> MALLAEHLLKPLPADKQIETGPFLEAVSHLPPFFDCLGSPVFTPIKDVISGNITKIKAVYDTNPAKFRTLQNILEVEKEMYGAEWPKVGATLALMWLKRGLRFIQVFLQSICDGERDENHPNLIRVNATKAYEMALKKYHGWIVQKIFQAALY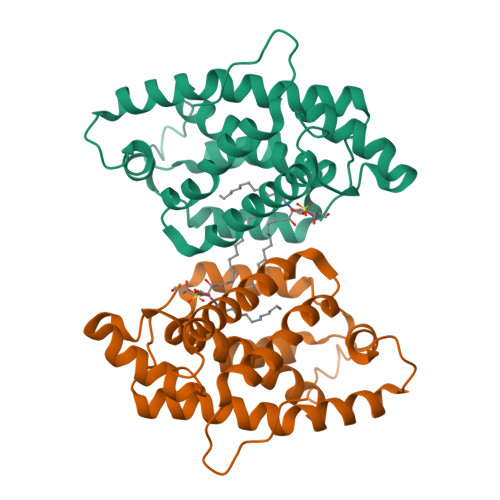AAPYKSDFLKALSKGQNVTEEECLEKIRLFLVNYTATIDVIYEMYTQMNAELNYKV> MGSSHHHHHHSSGENLYFQGSHMTATATSAKAAAPACPRFDDPVHAAADPRVDVERITPDPVWRTTCGTLYRSDSRGPAVVFEQGFLPKDVIDGQYDIESYVLGNQPSPYVSTT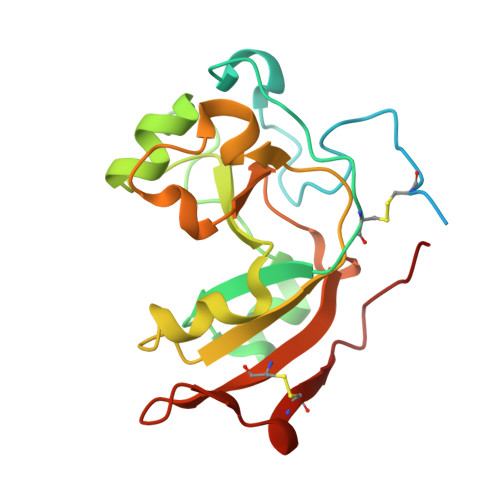YDHDLYKTWYKSGYNYYIDAPGGVDVNKTIGDRHKWADQVEVAFPGGIRTEFVIGVCPVDKKTRTEKMSECVGNPHYEPWH>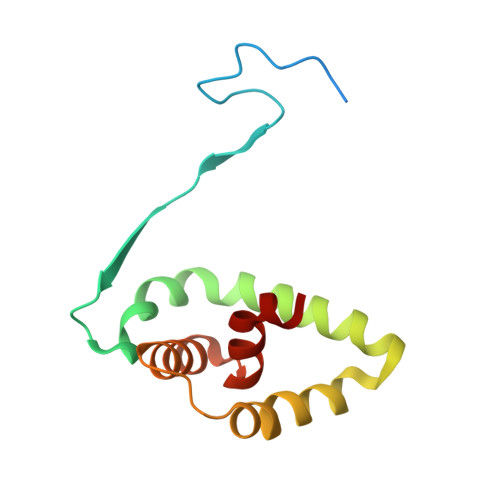 DRHHHHHHKLQHAPPWTEDCRKSTYPPSGPTYRGAVPWYTINLDLPPYKRWHELMLDKAPMLKVIVNSLKNMINTFVPSGKVMQVVDEKLPGLLGNFPGPFEEEMKGIAAVTDIPLGEIISFNIFYELF>[2x]NVLTVYSPYQSNLIRPILNEFEKQEHVKIEIKHGSTQVLLSNLHNEDFSERGDVFMGGVLSETIDHPEDFVPYQDTSVTQQLEDYRSN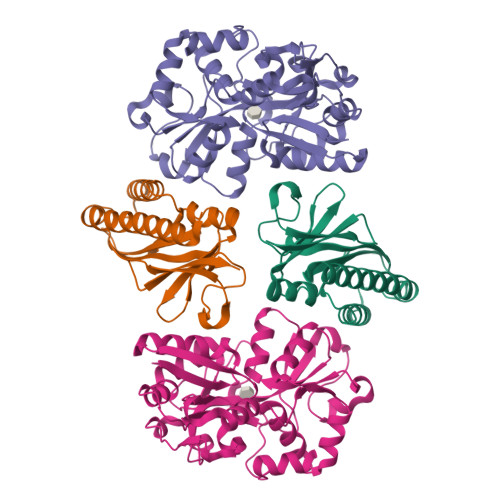NKYVTSFLLMPTVIVVNSDLQGDIKIRGYQDLLQPILKGKIAYSNPNTTTTGYQHMRAIYSMHHRVSDVHQFQNHAMQLSKTSKVIEDVAKGKYYAGLSYEQDARTWKNKGYPVSIVYPIEGTMLNVDGIALVKNAHPHPKRKKLVQYLTSRSVQQRLVAEFDAKSIRKDVSEQSDQSIENLKNIPLIPKSKLPDIPHHKFLEMIQ;>[2x]STIHQHVDESQSSLHHTEKQIQTFSTQHNNSFQELDLTNHHDVTATKRELLKLIHQQPATLYYELSGPNQFITNNYEHLNTKNMYLFSTHQLKFKNSTYMLKIYMANTPRLSEIKKDNRQFALIVDQYDNILYANDDRFTIGEKYRPQQFGFMNESVKLNHADHRLIIYKDI> MLDDRARMEAAKKEKVEQILAEFQLQEEDLKKVMRRMQKEMDRGLRLETHEEASVKMLPTYVRSTPEGSEVGDFLSLDLGGTNFRVMLVKVGEGEEGQWSVKTKHQMYSIPEDAMTGTAEMLFDYISECISDFLDKHQMKHKKLPLGFTFS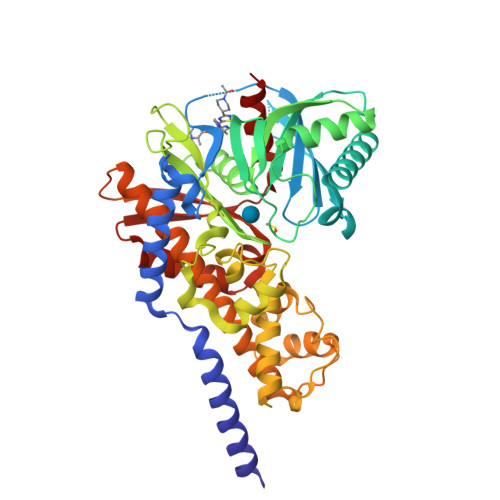FPVRHEDIDKGILLNWTKGFKASGAEGNNVVGLLRDAIKRRGDFEMDVVAMVNDTVATMISCYYEDHQCEVGMIVGTGCNACYMEEMQNVELVEGDEGRMCVNTEWGAFGDSGELDEFLLEYDRLVDESSANPGQQLYEKLIGGKYMGELVRLVLLRLVDENLLFHGEASEQLRTRGAFETRFVSQVESDTGDRKQIYNILSTLGLRPSTTDCDIVRRACESVSTRAAHMCSAGLAGVINRMRESRSEDVMRITVGVDGSVYKLHPSFKERFHASVRRLTPSCEITFIESEEGSGRGAALVSAVACK>[2x]VSVSEIRKAQRAEGPATILAIGTANPANCVEQSTYPDF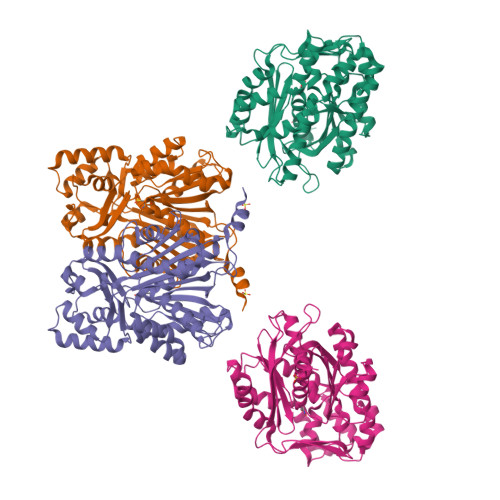YFKITNSEHKTELKEKFQRMCDKSMIKRRYMYLTEEILKENPNVCEYMAPSLDARQDMVVVEVPRLGKEAAVKAIKEWGQPKSKITHLIVCTTSGVDMPGADYQLTKLLGLRPYVKRYMMYQQGCFAGGTVLRLAKDLAENNKGARVLVVCSEVTAVTFRGPSDTHLDSLVGQALFGDGAAALIVGSDPVPEIEKPIFEMVWTAQTIAPDSEGAIDGHLREAGLTFHLLKDVPGIVSKNITKALVEAFEPLGISDYNSIFWIAQPGGPAILDQVEQKLALKPEKMNATREVLSEYGNMSSACVLFILDEMRKKSTQNGLKTTGEGLEWGVLFGFGPGLTIETVVLRSVAI> SLAPYASLTEIEHLVQSVCKSYRETCQL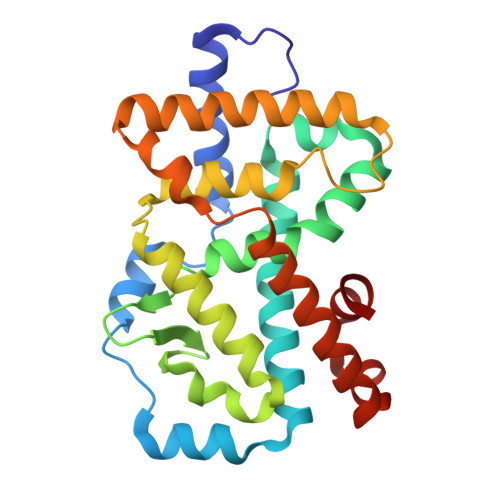RLEDLLRQRSNIFSREEVTGYQRKSMWEMWERCAHHLTEAIQYVVEFAKRLSGFMELCQNDQIVLLKAGAMEVVLVRMCRAYNADNRTVFFEGKYGGMELFRALGCSELISSIFDFSHSLSALHFSEDEIALYTALVLINAHRPGLQEKRKVEQLQYNLELAFHHHLCKTHRQSILAKLPPKGKLRSLCSQHVERLQIFQHLHPIVVQAAFPPLYKELFS>GARASVLSGGELDKWEKIRLRPGGKKQYKLKHIVWASRELERFAVNPGLLETSEGCRQILGQLQPSLQTGSEELRSLYNTIAVLYCVHQRIDVKDTKEALDKIEEEQNKSKKKAQQAAADTGNNSQVSQNY[12x];>FLGKIWPSHKGRPGNF[12x]

In immature virus particles, the Gag membrane-binding domain, MA, forms a hexameric protein lattice that undergoes structural transition, following cleavage, into a distinct, mature MA lattice. The MA domain is responsible for the recruitment of Gag to the host plasma membrane during virus assembly. MA forms a trimer that interacts with membranes in a phosphatidylinositol 4,5-bisphosphate (PtdIns(4,5)P2)-dependent manner through a highly basic region (HBR) and an amino-terminal myristate moiety. Here we show that released spacer peptide 2 (SP2), a conserved peptide of unknown function situated about 300 residues downstream of MA, binds MA to induce structural maturation.

However, we previously observed that this is not the case: a Gag mutant in which cleavage between MA and CA and cleavage between CA and SP1 are blocked (MA–SP1) exhibits an immature CA lattice and a mature MA lattice, suggesting that long-range interactions may be important for MA lattice maturation. We obtained reconstructions of the MA lattice from immature (PR−) virus particles at 5.8 Å, from mature virus particles at 3.8 Å and from MA–SP1 virus particles (in which MA also adopts a mature lattice) at 3.1 Å. In the mature MA lattice, the ordered loop between α-helix 1 and α-helix 2 sits at the centre of the inter-trimer interaction, forming a 230-Å2 interface with, in particular, α-helix 4 in its two-fold-related neighbour and a 90-Å2 interface including the 310 helix of another MA molecule. The loop between α-helix 1 and α-helix 2 overlaps with the previously described HBR of MA, and the structure revealed HBR binding into an acidic surface in the adjacent trimer: the positions of residues R20, K26 and K95 allow them to form inter-trimer salt bridges with E52, E73 or E74 and E55, respectively. Sandwiched between the two-fold-related neighbours is the ligand-bound side pocket where the two symmetry-related ligand densities come into close contact, bridged by residue R22. We found that, indeed, the six sequential C-terminal residues (GRPGNF) of SP2 could be confidently fitted into the cryo-EM density in a manner consistent with reconstructions of the mature MA lattice from WT, MA–SP1 and MA–NC particles. In the resulting model, bound SP2 adopted a largely extended conformation, with G11 at the top close to the viral membrane, and the C-terminal F16 at the base. The peptide is held in place by multiple interactions, including π-stacking between the backbone amides of SP2 R12 and P13 with MA W36 and H33, respectively, and a salt bridge between SP2 R12 and MA E73. A cleft consisting of residues L21, Y29, S77, T81 and T97 supports the binding of SP2 residues G14 and N15. SP2 seems to contribute to formation of the inter-trimer interactions in the mature MA lattice through a salt bridge between the C-terminal carbonyl and R22 in the two-fold-related MA molecule.>MLKFRTVHGGLRLLGIRRTSTAPAASPNVRRLEYKPIKKVMVANRGEIAIRVFRACTELGIRTVAIYSEQDTGQMHRQKADEAYLIGRGLAPVQAYLHIPDIIKVAKENNVDAVHPGYGFLSERADFAQACQDAGVRFIGPSPEVVRKMGDKVEARAIAIAAGVPVVPGTDAPITSLHEAHEFSNTYGFPIIFKAAYGGGGRGMRVVHSYEELEENYTRAYSEALAAFGNGALFVEKFIEKPRHIEVQILGDQYGNILHLYERDCSIQRRHQKVVEIAPAAHLDPQLRTRLTSDSVKLAKQVGYENAGTVEFLVDRHGKHYFIEVNSRLQVEHTVTEEITDVDLVHAQIHVAEGRSLPDLGLRQENIRINGCAIQCRVTTEDPARSFQPDTGRIEVFRSGEGMGIRLDNASAFQGAVISPHYDSLLVKVIAHGKDHPTAATKMSRALAEFRVRGVKTNIAFLQNVLNNQQFLAGTVDTQFIDENPELFQLRPAQNRAQKLLHYLGHVMVNGPTTPIPVKASPSPTDPVVPAVPIGPPPAGFRDILLREGPEGFARAVRNHPGLLLMDTTFRDAHQSLLATRVRTHDLKKIAPYVAHNFSKLFSMENWGGATFDVAMRFLYECPWRRLQELRELIPNIPFQMLLRGANAVGYTNYPDNVVFKFCEVAKENGMDVFRVFDSLNYLPNMLLGMEAAGSAGGVVEAAISYTGDVADPSRTKYSLQYYMGLAEELVRAGTHILCIKDMAGLLKPTACTMLVSSLRDRFPDLPLHIHTHDTSGAGVAAMLACAQAGADVVDVAADSMSGMTSQPSMGALVACTRGTPLDTEVPMERVFDYSEYWEGARGLYAAFDCTA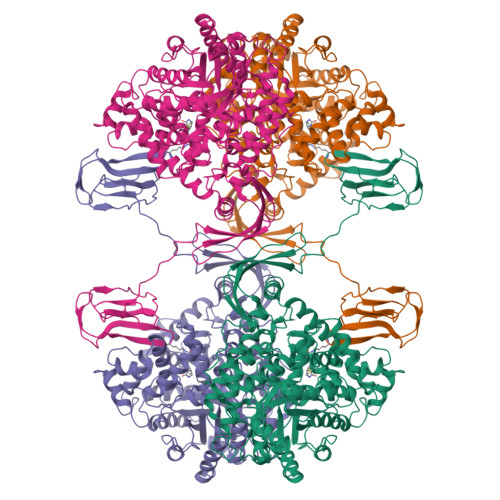TMKSGNSDVYENEIPGGQYTNLHFQAHSMGLGSKFKEVKKAYVEANQMLGDLIKVTPSSKIVGDLAQFMVQNGLSRAEAEAQAEELSFPRSVVEFLQGYIGVPHGGFPEPFRSKVLKDLPRVEGRPGASLPPLDLQALEKELVDRHGEEVTPEDVLSAAMYPDVFAHFKDFTATFGPLDSLNTRLFLQGPKIAEEFEVELERGKTLHIKALAVSDLNRAGQRQVFFELNGQLRSILVKDTQAMKEMHFHPKALKDVKGQIGAPMPGKVIDIKVVAGAKVAKGQPLCVLSAMKMETVVTSPMEGTVRKVHVTKDMTLEGDDLILEIE[4x]6-(5-bromo-2-methoxyphenyl)-9H-purin-2-amine 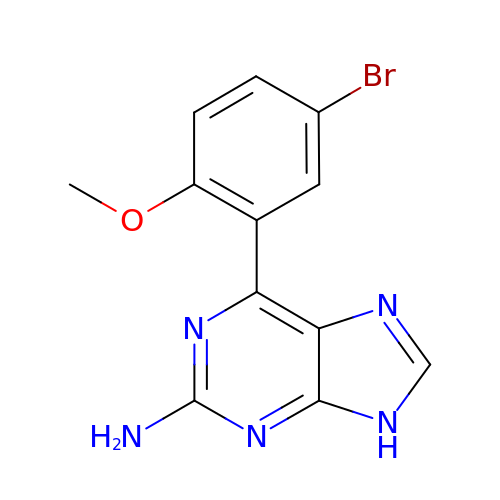| C12 H10 Br N5 O | KDNVOUMYSICLPF-UHFFFAOYSA-N> MGNLAGIMHRPDSEMAYVVNEQTVNIRLRTAKDDIVSVELLAGDPYSLRSLPTDEKFYQVPKQMTKIMSDGISDFWQVTVTEPKRRLAYAFLVTDMLGIQKIYSDKGFFKVADADLMDMNFYFRMPFFQTIDQYNAPEWVTDTVWYQIFPERFANGDVSNDPVGTKPWDSTDHPGREDFYGGDLQGILDHLDHLQELGISGIYLNPIFQAPSNHKYDTQDYMTVDPHFGDAKLFKQLVQAAHERGIRVMLDAVFNHIGDKSVQWQDVLKNEQASPYADWFHIHQFPATYTPTDNFEFAADATYDTFDYTPHMPKLNTSNPEVVDYLLNIATYWVKEFDIDAWRLDVANEIDHHFWRKFHDAMMALKPDFYILGEIWHTSQSWLVGDEFTAVMNYSYTGAILQYFLENESADALVQKMSHQLMLYRDATNRMMFNTVDSHDTPRLMTLAHEDKQLAKSIL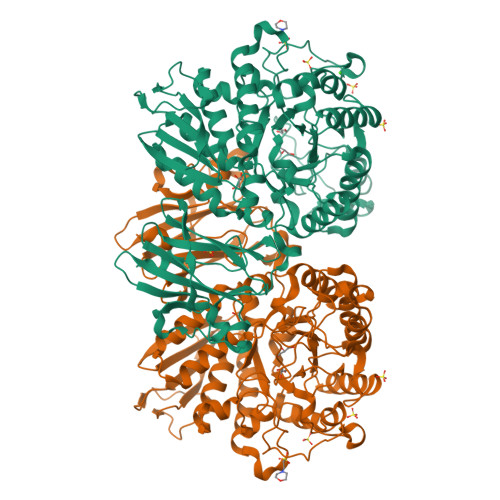TFTFMQPGVPSIYYGTEYGMTGENDPDDRKPMVWQPELQDHDLYDFMQKLVQVRRQVIAKLSDDKIIFDVIGERQIRLTREDNQTRIVGVFNNGTTDLTVAQPTSILLKTNQSETQLAPNDFMIWTEPVR> GMGFTIDIKSFLKPGEKTYTQRCRLFVGNLPTDITEEDFKRLFERYGEPSEVFINR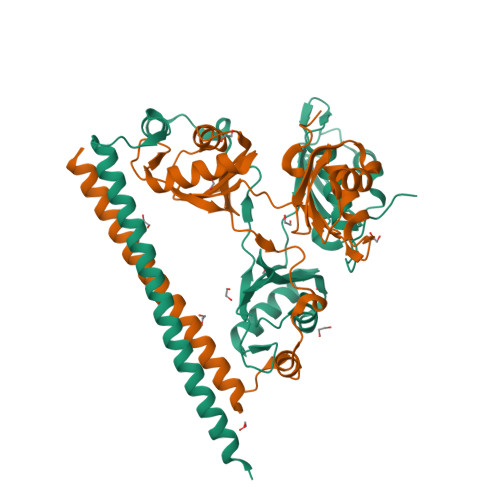DRGFGFIRLESRTLAEIAKAELDGTILKSRPLRIRFATHGAALTVKNLSPVVSNELLEQAFSQFGPVEKAVVVVDDRGRATGKGFVEFAAKPPARKALERCGDGAFLLTTTPRPVIVEPMEQFDDEDGLPEKLMQKTQQYHKEREQPPRFAQPGTFEFEYASRWKALDEMEKQQREQVDRNIREAKEKLEAEMEAARHEHQLMLM;> MEGLTIDLKNFRKPGEKTFTQRSRLFVGNLPPDITEEEMRKLFEKYGKAGEVFIHKDKGFGFIRLETRTLAEIAKVELDNMPLRGKQLRVRFACHSASLTVRNLPQYVSNELLEEAFSVFGQVERAVVIVDDRGRPSGKGIVEFSGKPAARKALDRCSEGSFLLTTFPRPVTVEPMDQLDDEEGLPEKLVIKNQQFHKEREQPPRFAQPGSFEYEYAMRWKALIEMEKQQQDQVDRNIKEAREKLEMEMEAARHEHQVMLM> GSAKNSSNRMYMEKSQTELGDLSDTLLSKVDDLQDVIEIMRKDVAERRSQPAKKKLETVSKDLENAQADVLKLQEFIDTEKPHWKKTWE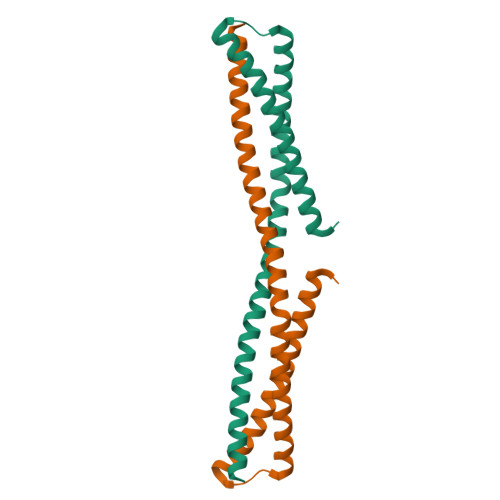AELDKVCEEQQFLTLQEELILDLKEDLGKALETFDLIKLCCEEQEKNPSRSK> MGLVPECFITELVERDLKEGKYAKLVTRFPPEPNGYLHIGHARSIVLNFGLAQDYGGECNLRFDDTNPETEKEEYARAIEEDVRWLGFRPTRVLYASDYFETMYQCALVLIQEGKAYVDDLPEEE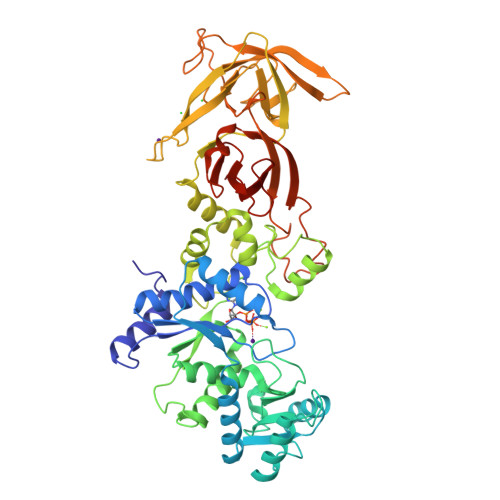MSELRAQGKPSPYRERSVEENLELFERMRRGEFPTGSRVLRAKIDPAHPNFKLRDPVLYRIVHAPHYHVGDRWVIYPMYDFAHPLEDFIEGVTHSLCTLEFENNRTVYDWVIENLKGKCGLPTSPRPHQYEFARLDLSHTVLSKRKLIKLVEGGYVSGWDDPRLPTLRGLRRRGVRPEAIVEFVRKTGISRNEAQIEMDLFEEVVRDDLNPIAPRVLGVVDPLKVVLTNYEGEEWIEAPYWPRDIPKEGTRPLPFSPELYIERTDFSLNPPKGWKRLAPGQRVRLRHAYVIELEDVVEEGGEVRLLKARIVPGTLGANPEDGVRPKGVIHWVSARHALPVEFRLYGRLFRTKDPEEGGDFLQNLNPEALVVKRGFIEPSVAQDPEDTRYQLERLGYFWRDPVDSRPEALVMNRIVPLKEGYRV dTDP-4,6-dideoxy-4-formamido-glucose | C17 H27 N3 O15 P2 | 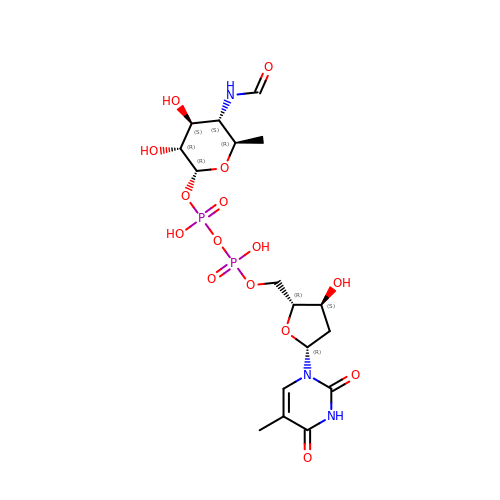QULUVRDLMBXPHO-GJSHGOAISA-N>MEIKLEEILKKQPLYSGKAKSIYEIDDDKVLIEFRDDITAGNGAKHDVKQGKGYLNALISSKLFEALEENGVKTHYIKYIEPRYMIAKKVEIIPIEVIVRNIAAGSLCRRYPFEEGKELPFPIVQFDYKNDEYGDPMLNEDIAVALGLATREELNKIKEIALKVNEVLKKLFDE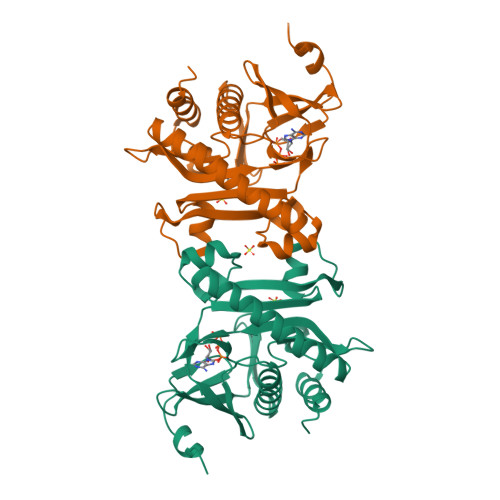KGIILVDFKIEIGKDREGNLLVADEISPDTMRLWDKETRDVLDKDVFRKDLGDVIAKYRIVAERLGLL[2x]>[7x]AEPVYPDQLRLFSLGQGVCGDKYRPVNREEAQSVKSNIVGMMGQWQISGLANGWVIMGPGYNGEIKPGTASNTWCYPTNPV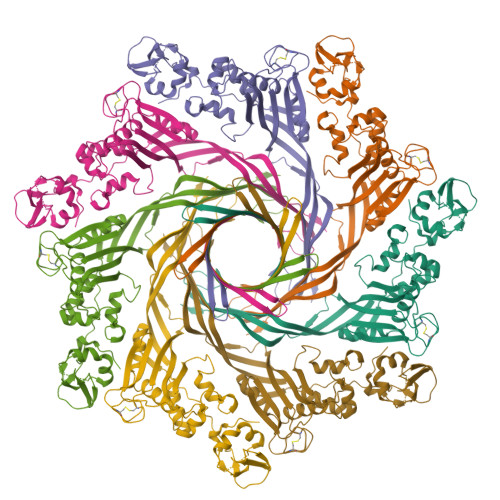TGEIPTLSALDIPDGDEVDVQWRLVHDSANFIKPTSYLAHYLGYAWVGGNHSQYVGEDMDVTRDGDGWVIRGNNDGGCDGYRCGDKTAIKVSNFAYNLDPDSFKHGDVTQSDRQLVKTVVGWAVNDSDTPQSGYDVTLRYDTATNWSKTNTYGLSEAVTTKNAFKWPLVGETELSIEIAANQSWASQNGGSTTTSLSQSVRPTVPARSKIPVKIELYKADISYPYEFKADVSYDLTLSGFLRWGGNAWYTHPDNRPNWNHTFVIGPYKDKASSIRYQWDKRYIPGEVKWWDWNWTIQQNGLSTMQNNLARVLRPVRAGITGDFSAESQFAGNIEIGAPVPLAA(2S)-2-[(2-azanyl-4-oxidanylidene-3H-pteridin-7-yl)carbonylamino]-3-(4-fluorophenyl)propanoic 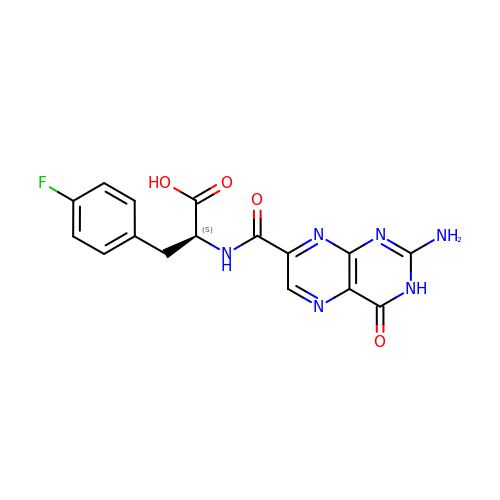acid | C16 H13 F N6 O4 | AGGHEPSDSCKUEM-VIFPVBQESA-N> GPLGSPNSEEEASVSVWDEEEDGATFTVTSRQYRPLDPLAPLPPPRSSRRLRAGTLEALVRHLLDARTAGADMMFTPALLATHRAFTSTPALFGLVADRLEALESYPPGELERTTGVAISVLSTWLASHPEDFGSEVKGQLDRLESFLLRTGYAAREGVVGGSADLIRNLRARVDPRAPDLPKPLAL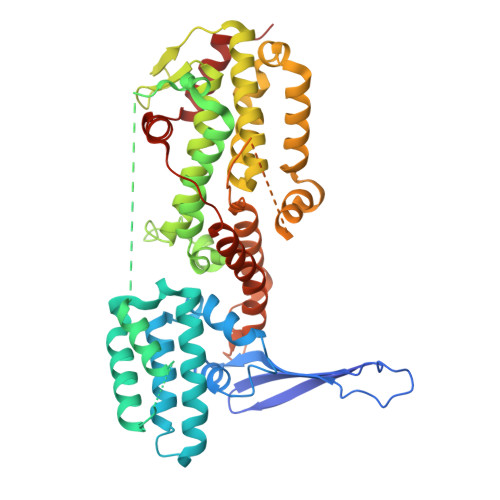PGDSPADPTDVLVFLADHLAEQLTLLDAELFLNLIPSQCLGGLWGHRDRPGHSHLCPSVRATVTQFNKVAGAVVSSVLGATSIGEGPREVTVRPLRPPQRARLLEKWIRVAEECRLLRNFSSVYAVVSALQSSPIHRLRAAWGETTRDSLRVFSSLCQIFSEEDNYSQSRELLTQEVKPQPPVEPHSKKAPRSGFRGGGVVPYLGTFLKDLVMLDAASKDELENGYINFDKRRKEFAILSELLRLQKECRGYDLRPNSDIQQWLQGLQPLTEAQSHRVSCEVEPPG>SSPPVVDTVHGKVLGKFVSLEGFAQPVAIFLGIPFAKPPLGPLRFTPPQPAEPWSFVKNATSYPPMCTQDPKAGQLLSELFTNRKENIPLKLSEDCLYLNIYTPADLTKKNRLPVMVWIHGGGLMVGAASTYDGLALAAHENVVVVTIQYRLGIWGFFSTGDEHSRGNWGHLDQVAALRWVQDNIASFGGNPGSVTIFGESAGGESVSVLVLSPLAKNLFHRAISESGVALTSVLVKKGDVKPLAEQIAITAGCKTTTSAVMVHCLRQKTEEELLETTLKMKFLSLDLQGDPRESQPLLGTVIDGMLLLKTPEELQAERNFHTVPYMVGINKQEFGWLIPMLMSYPLSEGQLDQKTAMSLLWKSYPLVCIAKELIPEATEKYLGGTDDTVKKKDLFLDLIADVMFGVPSVIVARNHRDAGAPTYMYEFQYRPSFSSDMKPKTVIGDHGDELFSVFGAPFLKEGASEEEIRLS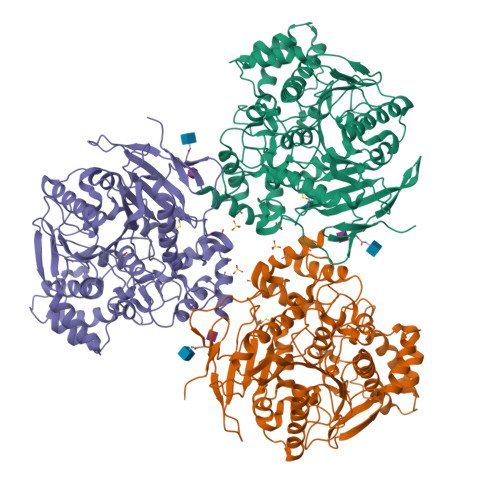KMVMKFWANFARNGNPNGEGLPHWPEYNQKEGYLQIGANTQAAQKLKDKEVAFWTNLFAK[12x]>MAHHHHHHMTRSETGRPSRRAFVTGLTGFTGRYMAERLQAAGYDVWGTVAPGTPRPADPAFAQCTLLPVDLLDAEAMRAAAADARPDAVVHLAARAHVAQDEPSQTYAVNIVGTRNLLAALSGLDRRPSAVLLASSANIYGNSTAGVLDETVAPAPANDYAVSKLAMEYAAKLWADRLPIVIARPFNYTGVGQSDAYLLPKLVAHYARNAPRISLGNLDVSRDFSDVRDVTAAYLKLIEAAPAGETFNVCSERAYSLKEVLAMLSRI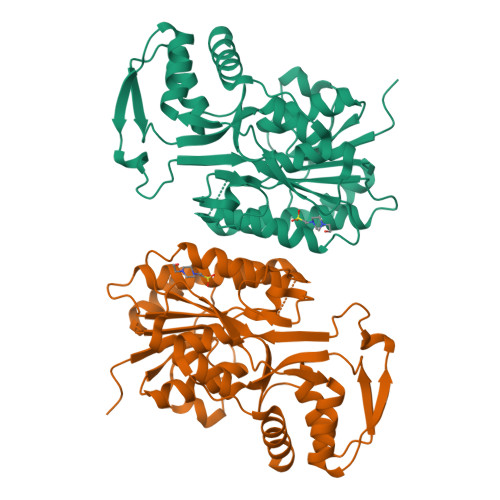AGYVIDVTIDPRFVRHNEVKSLSGSRDKLRRAVGELPVTPLDETLRWMVDAMRAAPPGHAAG[2x]>SGVSSPAPCPAPCACDLDGGADCSGKGLVTVPDGLSVFTHSLDLSMNNITKLPEGAFKGFPYLEELRLAGNDLSIIHPMALSGLKELKVLTLQNNQLKTVPSESLKGLVSLQSLRLDANHIVTVPEDSFEGLVQLRHLWLDDNSLTEVPIRPLSNLPSLQALTLALNKISHIPDYAFSNLSSLVVLHLHNNKIRTLGPHCFHGLDNLEALDLNYNNLIDFPDSIRSLPNLKELGFHSNSITIIPDGAFVKNPLLRTIHLYDNPLSFVGNSAFQNLSDLHFLIIRGASN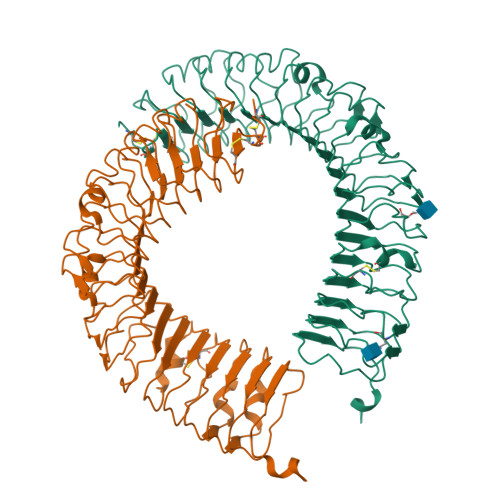VQWFPNLTGTNNLESLTLTGTKIRSIPIKFCQEQKMLRTLDLSYNEISALVGFEGCSSLEEVYLQNNQIQEVQNETFQGLAALRMLDLSRNRIHTIHKEAFVTLKALTNLDLSFNDLTAFPTAGLHGLNQLKLTGNPNFKETLT[2x]> QDRYLQDKKYIEFYVIVDNRMYRYYNNDKPAIKIKVYEMINAVNTKFRPLKIHIALIGLEIWSNKDKFEVKPAASVTLKSFGEWRETVLLPRKRNDNAQLLTGIDFNGNTVGRAYIGSLCKTNESVAIVQDYNRRISLVASTITHELGHNLGIHHDKASCICIPGPCIMLKKRTAPAFQFSSCSIREYRE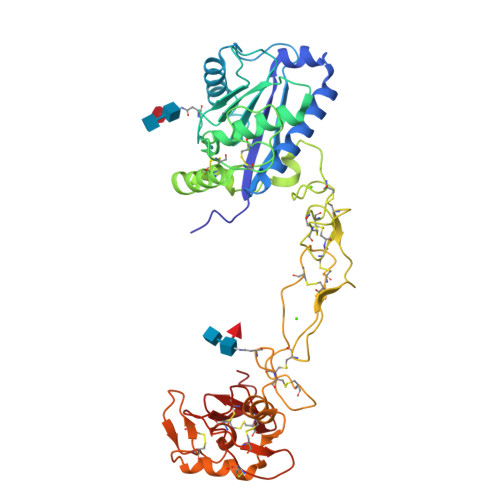YLLRDRPQCILNKPLSTDIVSPPICGNYFVEVGEECDCGSPQACQSACCNAATCQFKGAETECRVAKDDCDLPELCTGQSAECPTDSLQRNGHPCQNNQSYCYNGTCPTLTNQCITLLGPHFTVSPKGCFNLNMRGDDGSFCRMEDGTKIPCAAKDVKCGRLYCTEKNTMSCLIPPNPDGIMAEPGTKCGDGMVCSKGQCVDVQTAY> STSQKATYTDDFVLYRGDDFIEIIIDEKYLNKKVKILLDNDTIFNGILKDTSIFIPVKE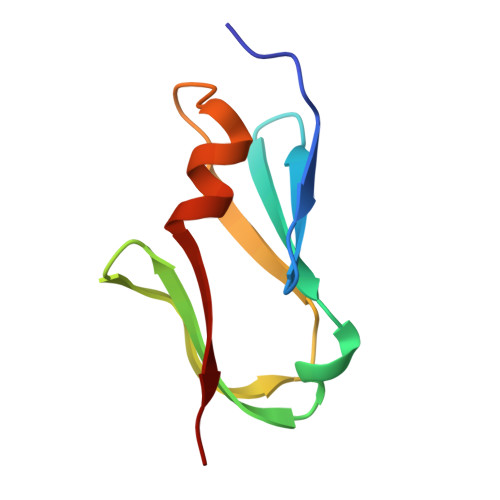QIDLEELAKHISILPEG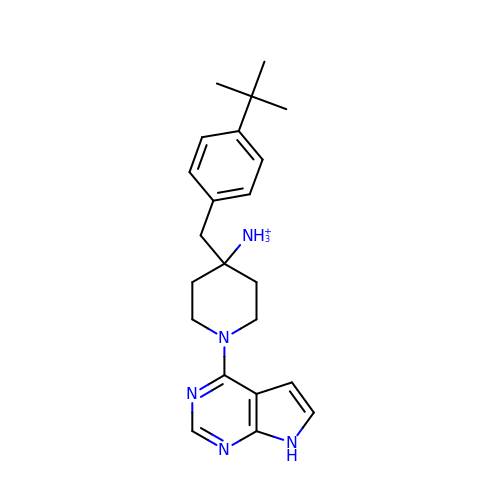4-(4-tert-butylbenzyl)-1-(7H-pyrrolo[2,3-d]pyrimidin-4-yl)piperidin-4-aminium | C22 H30 N5 | SNNUMARRAFQOGY-UHFFFAOYSA-O> LSTVSGSVAKVSSEKLAEKPVANIMDALQGQVAGMQVMTTSGDPTAVASVEIHGTGSLGASSAPLYIVDGMQTSLDVVATMNPNDFESMSVLKDASATSIYGARAANGVVFIQTKKGKMSERGRITFNASYGISQILNTKPLDNMMTGDELLDFQVKAGFWGNNQTVQKVKDMILAGAEDLYGNYDSLKDEYGKTLFPVDFNHDADWLKALFKTAPTSQGDISFSGGSQGTSYYASIGYFDQEGMAREPANFKRYSGRLNFESRINEWLKVGANLSGAIANRRSADYFGKYYMGSGTFGVLTMPRYYNPFDVNGDLADVYYMYGATRPSMTEPYFAKMRPFSSESHQANVNGFAQITPIKGLTLKAQAGVDITNTRTSSKRMPNNPYDSTPLGERRERAYRDVSKSFTNTAEYKFSIDEKHDLTALMGHEYIEYEGDVIGASSKGFESDKLMLLSQGKTGNSLSLPEHRVAEYAYLSFFSRFNYGFDKWMYIDFSVRNDQSSRFGSNNRSAWFYSVGGMFDIYNKFIQESN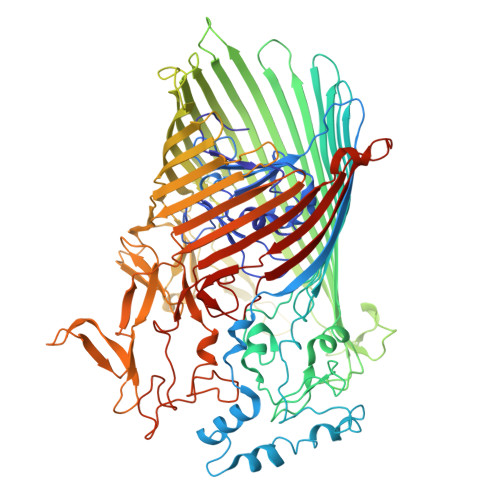WLSDLRLKMSYGTTGNSEIGNYNHQALVTVNNYTEDAMGLSISTAGNPDLSWEKQSQFNFGLAAGAFNNRLSAEVDFYVRTTNDMLIDVPMPYISGFFSQYQNVGSMKNTGVDLSLKGTIYQNKDWNVYASANFNYNRQEITKLFFGLNKYMLPNTGTIWEIGYPNSFYMAEYAGIDKKTGKQLWYVPGQVDADGNKVTTSQYSADLETRIDKSVTPPITGGFSLGASWKGLSLDADFAYIVGKWMINNDRYFTENGGGLMQLNKDKMLLNAWTEDNKETDVPKLGQSPQFDTHLLENASFLRLKNLKLTYVLPNSLFAGQNVIGGARVYLMARNLLTVTKYKGFDPEAGGNVGKNQYPNSKQYVAGIQLSF>[2x]GALSPGGTKQKYKEVVDIEAQRRLNDLAREARIRRAQQAVLRKELIATSTNVIKSEISLRILASECHLTLNGIVEAEAQYKMGGLPKSRLPKIKHPMIVTKWVDYSNKHGFSYQLSTEDIGVLFNNGTTVLRLADAEEFWYISYDDREGWVASHYLLSEKPRELSRHLEVVDFFAKYMKANLSRVSTFGREEYHKDDVFLRRYTRYKPFVMFELSDGTFQFNFKDHHKMA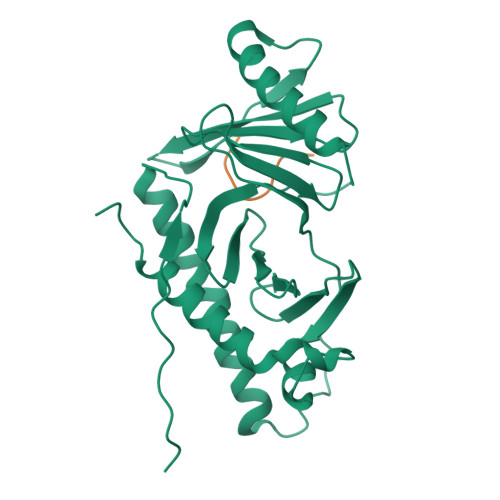ISDGGKLVTYISPSHESTTYPLVEVLKYGEIPGYPESNFREKLTLIKEGLKQKSTIVTVD;>[2x]RARIERARSIEGAVQVSKGTG(2S,3R)-N~4~-[(1S)-1-(dimethylcarbamoyl)-2,2-dimethylpropyl]-N~1~,2-dihydroxy-3-(2-methylpropyl)butanediamide 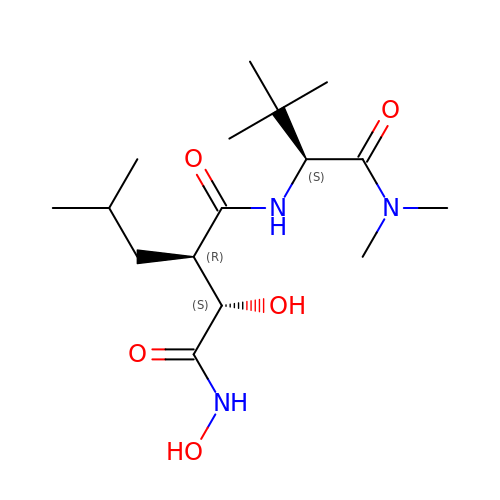| C16 H31 N3 O5 | USHCFFHZEHRVBD-GRYCIOLGSA-N> MSRSKRDNNFYSVEIGDSTFTVLKRYQNLKPIGSGAQGIVCAAYDAILERNVAIKKLSRPFQNQTHAKRAYRELVLMKCVNHKNIIGLLNVFT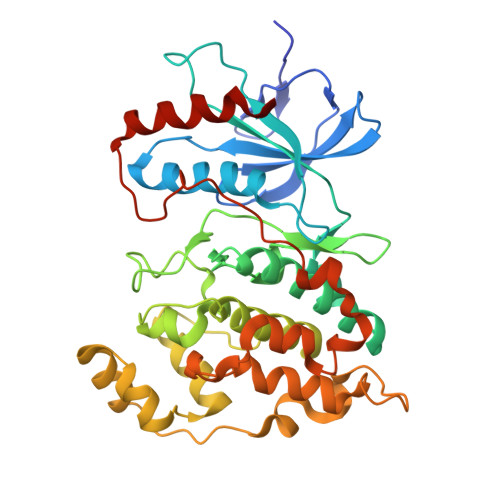PQKSLEEFQDVYIVMELMDANLCQVIQMELDHERMSYLLYQMLCGIKHLHSAGIIHRDLKPSNIVVKSDCTLKILDFGLARTAGTSFMMEPEVVTRYYRAPEVILGMGYKENVDLWSVGCIMGEMVCHKILFPGRDYIDQWNKVIEQLGTPCPEFMKKLQPTVRTYVENRPKYAGYSFEKLFPDVLFPADSEHNKLKASQARDLLSKMLVIDASKRISVDEALQHPYINVWYDPSEAEAPPPKIPDKQLDEREHTIEEWKELIYKEVMDLEHHHHHH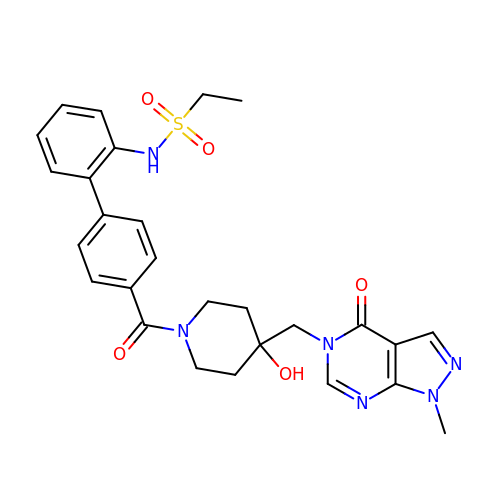~{N}-[2-[4-[4-[(1-methyl-4-oxidanylidene-pyrazolo[3,4-d]pyrimidin-5-yl)methyl]-4-oxidanyl-piperidin-1-yl]carbonylphenyl]phenyl]ethanesulfonamide | C27 H30 N6 O5 S | RLNXXNBZMTXHGJ-UHFFFAOYSA-N>MKDEVALLAAVTLLGVLLQAYFSLQVISARRAFR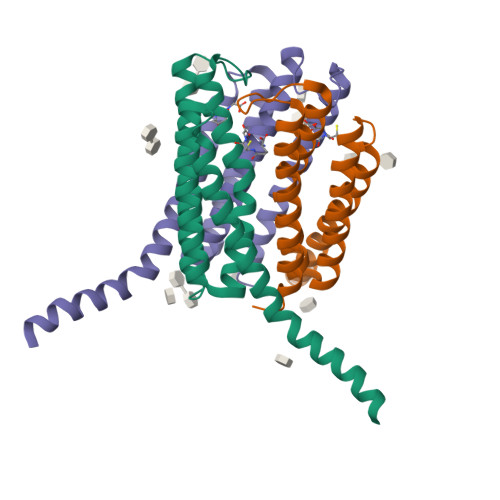VSPPLTTGPPEFERVYRAQVNCSEYFPLFLATLWVAGIFFHEGAAALCGLVYLFARLRYFQGYARSAQLRLAPLYASARALWLLVALAALGLLAHFLPAALRAALLGRLRTLLPWAHHHHHH[12x]>[2x]MEFKDFPLKPEILEALHGRGLTTPTPIEAAALPLALEGKDLIGQARTGTGKTLAFALPIAERLAPSQERGRKPRALVL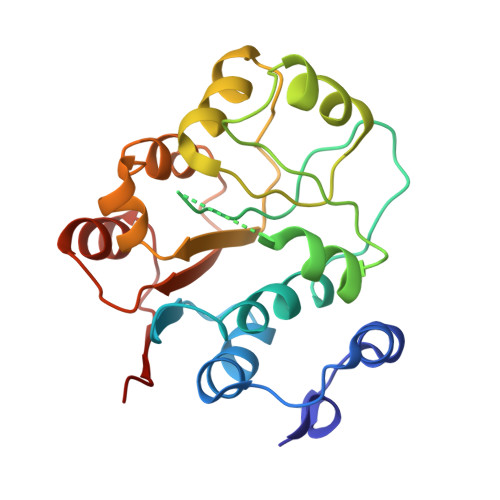TPTRELALQVASELTAVAPHLKVVAVYGGTGYGKQKEALLRGADAVVATPGRALDYLRQGVLDLSRVEVAVLDEADEMLSMGFEEEVEALLSATPPSRQTLLFSATLPSWAKRLAERYMKNPVLINVIK> VSEIKTLVTFFGGTGDLAKRKLYPSVFNLYKKGYLQKHFAIVGTARQALNDDEFKQLVRDSIKDFTDDQA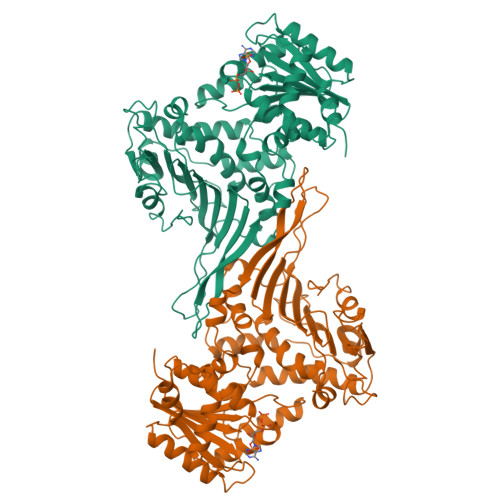QAEAFIEHFSYRAHDVTDAASYAVLKEAIEEAADKFDIDGNRIFYMSVAPRFFGTIAKYLKSEGLLADTGYNRLMIEKPFGTSYDTAAELQNDLENAFDDNQLFRIDHYLGKEMVQNIAALRFGNPIFDAAWNKDYIKNVQVTLSEVLGVEERAGYYDTAGALLDMIQNNTMQIVGWLAMEKPESFTDKDIRAAKNAAFNALKIYDEAEVNKYFVRAQYGAGDSADFKPYLEELDVPADSKNNTFIAGELQFDLPRWEGVPFYVRSGKRLAAKQTRVDIVFKAGTFNFGSEQEAQEAVLSIIIDPKGAIELKLNAKSVEDAFNTRTIDLGWTVSDEDKKNTPEPYERMIHDTMNGDGSNFADWNGVSIAWKFVDAISAVYTADKAPLETYKSGSMGPEASDKLLAANGDAWVFKG> MPDFLGHAENPLREEEWARLNETVIQVARRSLVGRRILDIYGPLGAGVQTVPYDEFQGVSPGAVDIVGEQETAMVFTDARKFKTIPIIYKDFLLHWRDIEAARTHNMPLDVSAAAGAA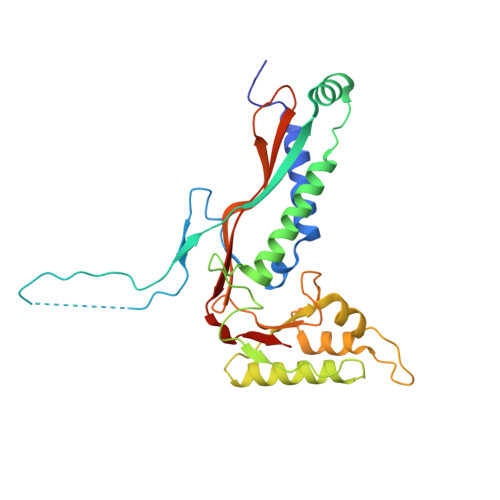ALCAQQEDELIFYGDARLGYEGLMTANGRLTVPLGDWTSPGGGFQAIVEATRKLNEQGHFGPYAVVLSPRLYSQLHRIYEHHHVLEIETIRQLASDGVYQSNRLRGESGVVVSTGRENMDLAVSMDMVAAYLGASRMNHPFRVLEALLLRIKHPDAICTLEGAGATERR> MKIRSQVGMVLNLDKCIGCHTCSVTAKNVWTSREGVEYAWFNNVETKPGQGFPTDWENQEKYKGGWIRKINGKLQPRMGNRAMLLGKIFANPHLPGIDDYYEPFDFDYQNLHTAPEGSKSQPIARPRSLITGERMAKIEKGPNWEDDLGGEFDKLAKDKNFDNIQKAMYSQFENTFMMYLPRLCEHCLNPACVATCPSGAIYKREEDGIVLIDQDKCRGWRMCITGCPYKKIYFNWKSGKSEKCIFCYPRIEAGQPTVCSET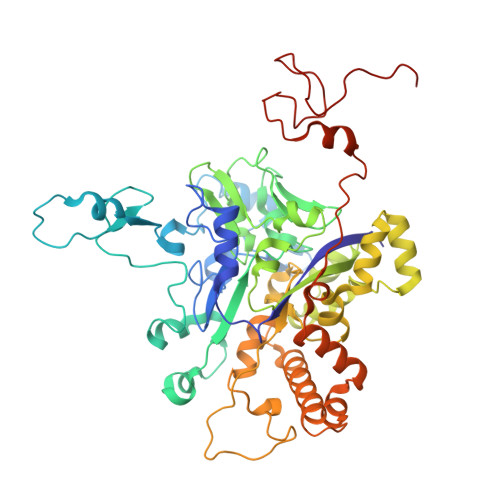CVGRIRYLGVLLYDADAIERAASTENEKDLYQRQLDVFLDPNDPKVIEQAIKDGIPLSVIEAAQQSPVYKMAMEWKLALPLHPEYRTLPMVWYVPPLSPIQSAADAGELGSNGILPDVESLRIPVQYLANLLTAGDTKPVLRALKRMLAMRHYKRAETVDGKVDTRALEEVGLTEAQAQEMYRYLAIANYEDRFVVPSSHRELAREAFPEKNGCGFTFGDGCHGSDTKFNLFNSRRIDAIDVTSKTEPHP> MSNWVMQEENKQGNLTPLFEELLQQCPPGGQNKTAHMVSAYQLAQGNWMPTSCHVFMGTISARRTKTHPYEAYVKLRELVEEHKMKTLCPGSSLGKHNDWIIGKIKYQGNLRTKHMLNPGKVAEQ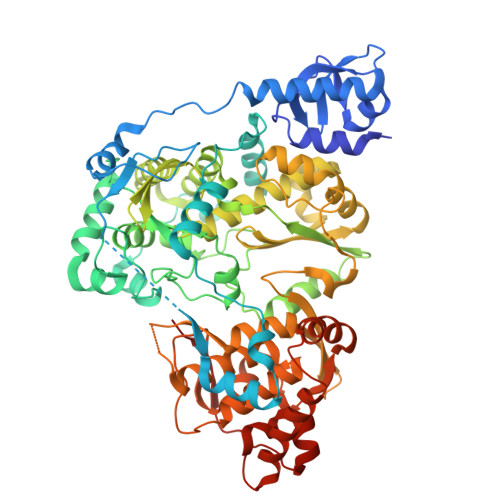LCREGHRHNVYNKTIGSVMTATGIRLEKLPVVRAQTDTTNFHQAIRDKIDKEENLQTPGLHKKLMEVFNALKRPELESSYDAVEWEELERGINRKGAAGFFERKNIGEILDSEKNKVEEIIDNLKKGRNIKYYETAIPKNEKRDVNDDWTAGDFVDEKKPRVIQYPEAKTRLAITKVMYKWVKQKPVVIPGYEGKTPLFQIFDKVKKEWDQFQNPVAVSFDTKAWDTQVTTKDLELIKDIQKYYFKKKWHKFIDTLTMHMTEVPVICADGEVYIRKGQRGSGQPDTSAGNSMLNVLTMVYAFCEATGVPYKSFDRVAKIHVCGDDGFLITERALGEKFASKGVQILYEAGKPQKITEGDKMKVAYQFDDIEFCSHTPIQVRWSDNTSSYMPGRNTTTILAKMATRLDSSGERGTIAYEKAVAFSFLLMYSWNPLIRRICLLVLSTELQVKPGKSTTYYYEGDPISAYKEVIGHNLFDLKRTSFEKLAKLNLSMSVLGAWTRHTSKRLLQDCVNMGVKEGNWLVNADRLVSSKTGNRYIPGEGHTLQGRGSSSHHHHHH> TFEYG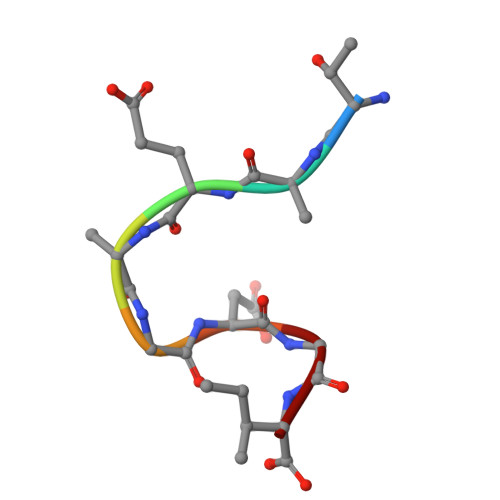DGI> MSTSWSDRLQNAADMPANMDKHALKKYRREAYHRVFVNRSLAMEKIKCFGFNMDYTLAVYKSPEYESLGFELTVERLVSIGYPQELLSFAYDSTFPTRGLVFDTLYGNLLKVDAYGNLLVCAHGFNFIRGPETREQYPNKFIQRDDTERFYILNTLFNLPETYLLACLVDFFTNCPRYTSCETGFKDGDL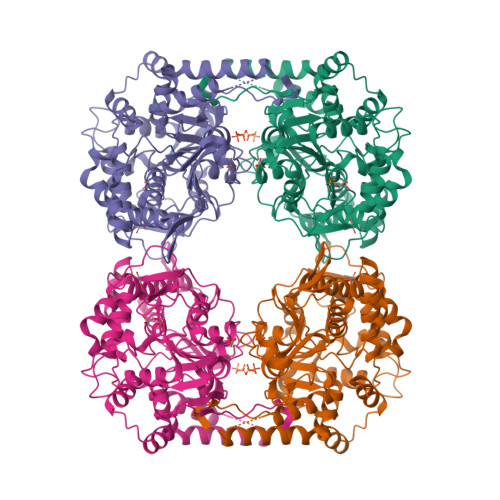FMSYRSMFQDVRDAVDWVHYKGSLKEKTVENLEKYVVKDGKLPLLLSRMKEVGKVFLATNSDYKYTDKIMTYLFDFPHGPKPGSSHRPWQSYFDLILVDARKPLFFGEGTVLRQVDTKTGKLKIGTYTGPLQHGIVYSGGSSDTICDLLGAKGKDILYIGDHIFGDILKSKKRQGWRTFLVIPELAQELHVWTDKSSLFEELQSLDIFLAELYKHLASSSNERPDISSIQRRIKKVTHDMDMCYGMMGSLFRSGSRQTLFASQVMRYADLYAASFINLLYYPFSYLFRAAHVLMPHESTVEHTHVDINEMESPLATRNRTSVDFKDTDYKRHQLTRSISEIKPPNL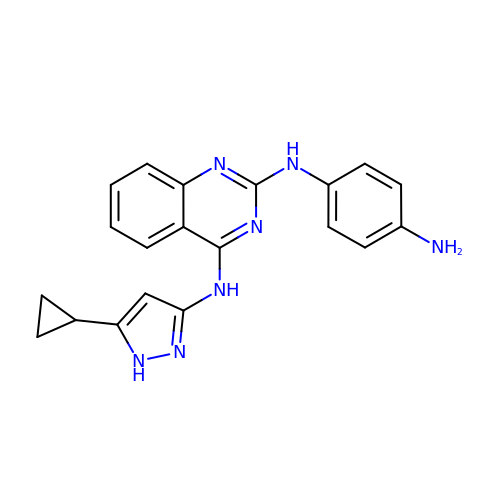N~2~-(4-aminophenyl)-N~4~-(5-cyclopropyl-1H-pyrazol-3-yl)quinazoline-2,4-diamine | C20 H19 N7 | CWKAMSLBSGZMJZ-UHFFFAOYSA-N>MGRDLRDNETWWYNPSIVVHPHWREFDQVPDAVYYSLGIFIGICGIIGCGGNGIVIYLFTKTKSLQTPANMFIINLAFSDFTFSLVNGFPLMTISCFLKKWIFGFAACKVYGFIGGIFGFMSIMTMAMISIDRYNVIGRPMAASKKMSHRRAFIMIIFVWLWSVLWAIGPIFGWGAYTLEGVLCNCSFDYISRDSTTRSNILCMFILGFFGPILIIFFCYFNIVMSVSNHEKEMAAMAKRLNAKELRKAQAGANAEMRLAKISIVIVSQFLLSWSPYAVVALLAQFGPLE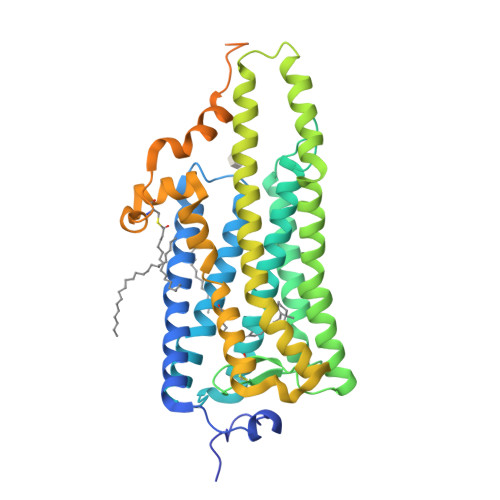WVTPYAAQLPVMFAKASAIHNPMIYSVSHPKFREAISQTFPWVLTCCQFDDKETEDDKDAETEIPAGESSDAAPSADAAQMKEMMAMMQKMQQQQAAYPPQGYAPPPQGYPPQGYPPQGYPPQGYPPQGYPPPPQGAPPQGAPPAAPPQGVDNQAYQA[2x]> MGTLTIDGKNKILATLTPTTIILHNVDPTADPTA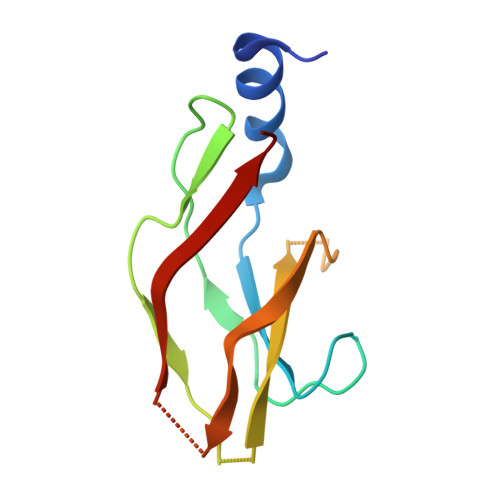NKVTQPVAIYFSEPDNGLIASEDTVNITVPASATVSHYSLWDANDKCVATGALSKPQFFAEEGIYVISSVSVDLNK>[2x]TAPSQVLKIRRPDDWHLHLRDGDMLKTVVPYTSEIYGRAIVMPNLAPPVTTVEAAVAYRQRILDAVPAG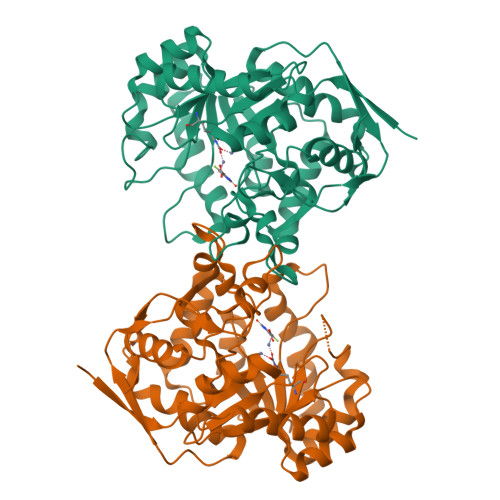HDFTPLMTCYLTDSLDPNELERGFNEGVFTAAKLYPANATTNSSHGVTSVDAIMPVLERMEKIGMPLLVHGEVTHADIDIFDREARFIESVMEPLRQRLTALKVVFEHITTKDAADYVRDGNERLAATITPQHLMFNRNHMLVGGVRPHLYCLPILKRNIHQQALRELVASGFNRVFLGTDSAPHARHRKESSCGCAGCFNAPTALGSYATVFEEMNALQHFEAFCSVNGPQFYGLPVNDTFIELVREEQQVAESIALTDDTLVPFLAGETVRWSVKQ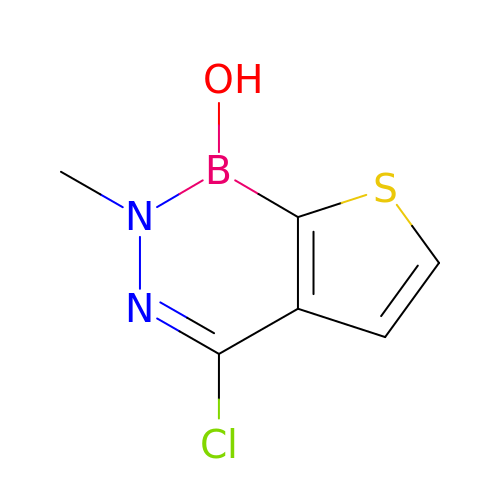4-chloro-2-methylthieno[2,3-d][1,2,3]diazaborinin-1(2H)-ol | C6 H6 B Cl N2 O S | UKYMGRYWPUJEOD-UHFFFAOYSA-N>[2x]MLGLKTSIIGRRVIYFQEITS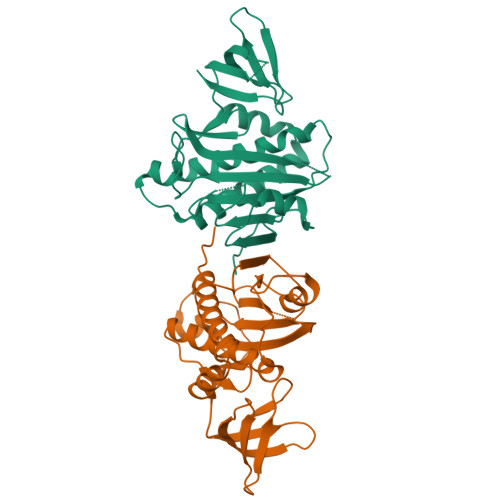TNEFAKTSYLEEGTVIVADKQTMGHGALNRKWESPEGGLWLSIVLSPKVPQKDLPKIVFLGAVGVVETLKEFSIDGRIKWPNDVLVNYKKIAGVLVEGKGDKIVLGIGLNVNNKVPNGATSMKLELGSEVPLLSVFRSLITNLDRLYLNFLKNPMDILNLVRDNMILGVRVKILGDGSFEGIAEDIDDFGRLIIRLDSGEVKKVIYGDVSLRFL> LT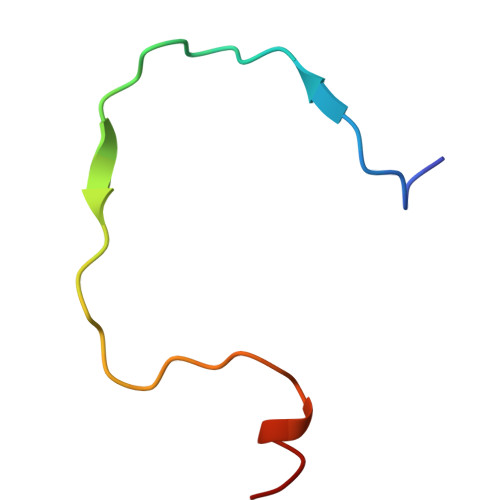ADNFQSPCALPEFDVTPPIDIPGEVKNMMELAEI>MHHHHHHMSSKQFKILVNEDYQVNVPSLPFRDVLQDIKYCYRNGFDGYVFVPEYRRDLVDCNRKDHYVIGVLGNG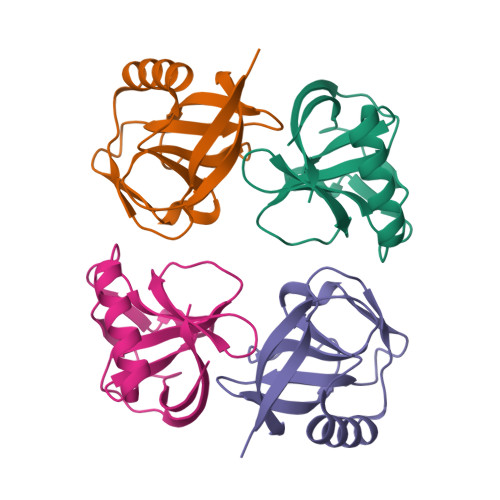ISDLKPVLLTEPSVMLQGFIVRADCNGVLEDFDLKIARTGNG[4x]> GSMGLSRVYSKLYKEAEKIKKWKVSTEAELRQKESKLQENRKIIEAQRKAIQ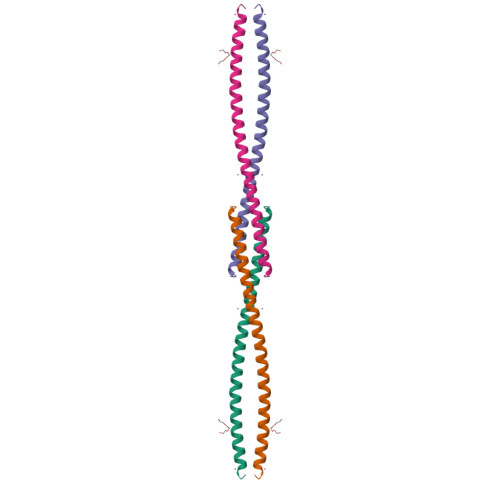ELQFGNEKVSLKLEEGIQENKDLIKE>IQTTAPPVKESSFVEKMKKTGRNIIVFYGSQTGTAEEFANRLSKDAHRYGMRGMSADPEEYDLADLSSLPEIDKSLVVFCMATYGEGDPTDNAQDFYDWLQETDVDLTGVKFAVFGLGNKTYEHFNAMGKYVDQRLEQLGAQRIFELGLGDDDGNLEEDFITWREQFWPAVCEFFGVEATGEESSIRQYELVVHEDMDVAKVYTGEMGRLKSYENQKPPFDAKNPFLAAVTANRKLNQGTERHLMHLELDISDSKIRYESGDHVAVYPANDSALVNQIGEILGADLDVIMSLNNLDEESNKKHPFPCPTTYRTALTYYLDITNPPRTNVLYELAQYASEPSEQEHLHKMASSSGEGKELYLSWVVEARRHILAILQDYPSLRPPIDHLCELLPRLQARYYAIASSSKVHPNSVHICAVAVEYEAKSGRVNKGVATSWLRAKEPAGENGGRALVPMFVRKSQFRLPFKSTTPVIMVGPGTGIAPFMGFIQERAWLREQGKEVGETLLYYGCRRSDEDYLYREELARFHKDGALTQLNVAFSREQAHKVYVQHLLKRDREHLWKLIHEGGAHIYVAGDARNMAKD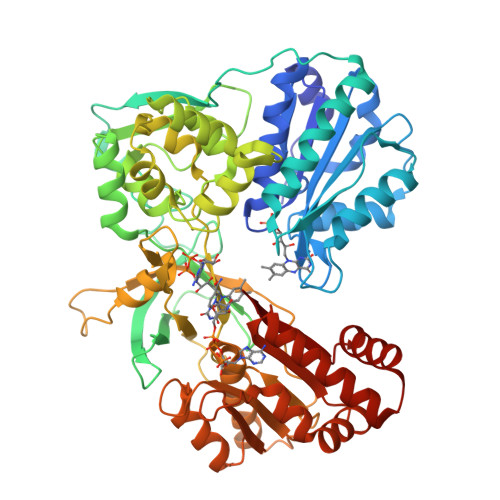VQNTFYDIVAEFGPMEHTQAVDYVKKLMTKGRYSLNVWS[2x]>MATEVTFFDELKIDNKVDIIGNNVRGELPNIWLQYGQFKLKASGGDGTYSWYSENTSIATVDASGKVTLNGKGSVVIKATSGDKQTVSYTIKAPSYMIKVDKQAYYADAMSICKNLLPSTQTVLSDIYDSWGAANKYSHYSSMNSITAWIKQTSSEQRSGVSSTYNLITQYPLPGVNVNTPNVYAVCVE[2x]

Intimin, an out membrane protein expressed by EHEC and EPEC, is required for intimate attachment to the host cell and formation of the A/E lesions. The binding of intimin to Tir mediates the adhesion between the pathogen and its host cell. The intimin of EHEC O157:H7 is of γ-type (designated intimin-γ), whereas that of EPEC is intimin-α. Here, we determined the crystal structures of Tir-binding domain of EHEC O157:H7 intimin at 2.8 Å, together with an Asn to Tyr mutant at amino acid 916 (IntN916Y) at 2.6 Å.

In this study, we solved the structure of EHEC Int188 and its mutant IntN916Y. Crystals of EHEC Int188 and IntN916Y diffract X-rays at 2.8 Å and 2.6 Å, respectively. R-free values were separately refined to 29.6% and 26.8%. These two versions of intimin (Int188 and IntN916Y) were crystallized in space group C2 and P212121, respectively. For the native version, Int188 consists of four molecules in the asymmetric unit while the IntN916Y is present in two molecules per asymmetric unit. Recent study have demonstrated that four important residues (S890, T909, N916 and N927) of EHEC intimin are essential for Tir recognition. It clearly indicates that these four residues locate in the Tir binding pocket which is formed by B, C, D β-sheets and the loop between D, E β-sheets. Int188 and IntN916Y behave completely the same at the level of higher structure (not shown). For the mutant, IntN916Y, the folding mode is completely the same as the native version, which indicates that this amino acid substitution fails to influence the alpha-C backbone in Int188.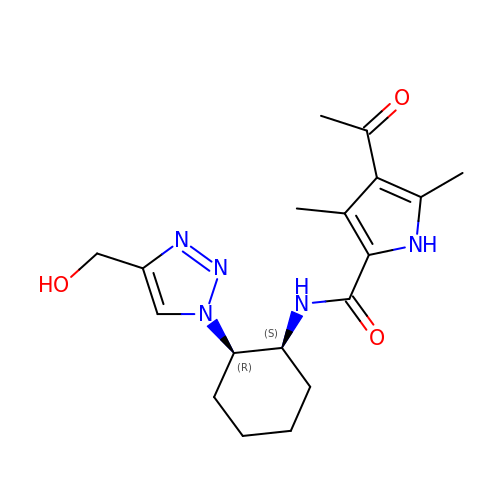4-ethanoyl-~{N}-[(1~{S},2~{R})-2-[4-(hydroxymethyl)-1,2,3-triazol-1-yl]cyclohexyl]-3,5-dimethyl-1~{H}-pyrrole-2-carboxamide | C18 H25 N5 O3 | TYCFYSXFDXDPGP-LSDHHAIUSA-N> MRLSWVIGGAQGTGIDTAANIFGNAVASAGYYIYGNREYYSNIKGRHSYFSLTISDKRVRSNTQKIDILVSFDAETVFQHFYDVKDILIYNKAVETTKIDAVQSMEPELAERIKDFLTKQGYETTVKGALEYASKNNVTLIPVNYDEIAKKVADEMKVPLSVTERVKNIVGITISYKLLGLDVNYLIEAINSTFKQDLYRKMNELAVKDSYDIVESRYNLKPSSKERRRFWLDGNTAVAIGKIYGGVRFQSYYPITPASDESVYIEAHQDVLMEDPITGDKKKGTIVVVQAEDELAAINMAIGAALTGVRAATATSGPGFSLMVEGLGWAGMNEVPVVITYYIRGGPSTGLPTRTAQSDLIFPIFAGHGEFPKIVLASGDHAEAFKDAIWALNLAEKYQTPVIHLVEKTLANSYSTIPYEELELDKLKAERGKIVESGDISYKRFKFTEDGISPRAFLGKATMYYTGDEHNEEGHISEDVVNRTMMYEKRMKKLEVADKEIPEESRVKIYGDLNSRNLIITWGSPTGVLRDILEESNFDFTLLQIRMFSPFPKNLVSKLMEGRDKIITVEGNYLAQTSLLVKMYTGKDVTNSILKWNGRPFLRDELEEAL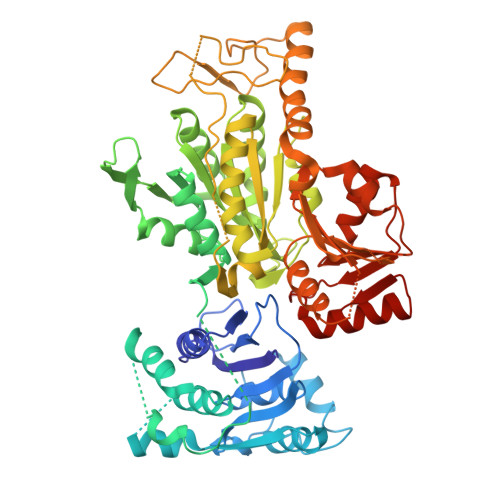IKVIKDGEKRVVLNGGI> VHITLDPDTANPWLILSEDRRQVRLGDTQQSIPGNEERFDSYPMVLGAQHFHSGKHYWEVDVTGKEAWDLGVCRDSVRRKGHFLLSSKSGFWTIWLWNKQKYEAGTYPQTPLHLQVPPCQVGIFLDYEAGMVSFYNITDHGSLIYSFSECAFTGPLRPFFSPGFNDGGKNTAPLTLCPL

Tripartite motif-containing protein 21 (TRIM21) is a member of the TRIM family, characterized by the presence of a RING finger domain, a B-box motif, a coiled-coil region, and a PRY-SPRY domain. Within the TRIM family, it has a unique role due to its specific binding to the Fc region of intracellular antibodies (AB) and thereby marking antibody-coated proteins or non-enveloped virus particles for proteasomal degradation. Central to the function of TRIM21 is the PRY-SPRY domain, which mediates interactions with immunoglobulin Fc regions. The PRY-SPRY domain contains a deep binding pocket, making it the most druggable and therefore most promising domain of the TRIM21 holoenzyme for therapeutic intervention.

Furthermore, we determined a high-resolution crystal structure of the potent ligand AL236 (1) bound to human TRIM21, which guided the design of AL244 (2), a tracer for a NanoBRET assay. Based on the discovered scaffold, we synthesized the representative ligand AL236 (1) and crystallized it under similar conditions as previously reported. Human TRIM21 PRY-SPRY domain at 10 mg mL−1 was co-crystallized with 500 µM AL236 (1) using the sitting-drop vapor diffusion method, with a reservoir solution containing 2.3 M sodium chloride and 0.1 M sodium citrate pH 3.5. Crystals in the space group P62 with a single monomer in the asymmetric unit, were grown with drop ratios of 0.1 μL protein, 0.1 μL reservoir solution at 20 °C. Before flash freezing in liquid nitrogen, the crystals were cryoprotected with 25% ethylene glycol dissolved in reservoir solution. The structure revealed that the ligand is occupying the whole pocket and binds by a combination of polar and nonpolar interactions. Similar to many fragments, it forms π-π interactions with the two tryptophans Trp381 and Trp383, as well as a polar interaction via its amide to the backbone of Leu371. Further structural analysis indicated that a promising strategy for an exit vector is to replace the terminal cyclohexyl group with a piperidine moiety and conjugate the BODIPY dye via a PEG linker to the piperidine nitrogen. This resulted in the tracer AL244 (2), which demonstrated desired properties. Initial measurements in life cells (intact mode) showed that AL236 (1) effectively displaced the tracer, with an EC50 of 197 nM. Under permeabilized conditions (lysed mode), we obtained a similar result (EC50: 297 nM), indicating a high cell permeability of this compound.> DSSDEASVSPIADNEREAVTLLLGYLEDKDQLDFYSGGPLKALTTLVYSDNLNLQRSAALAFAEITEKYVRQVSREVLEPILILLQSQDPQIQVAACAALGNLAVNNENKLLIVEMGGLEPLINQMMGDNVEVQCNAVGCITNLATRDDNKHKIATSGALIPLTKLAKSKHIRVQRNATGALLNMTHSEENRKELVNAGAVPVLVSLLSSTDPDVQYYCTTALSNIAVDEANRKKLAQTEPRLVSKLVSLMDSPSSRVKCQATLALRNLASDTSYQLEIVRAGGLPHLVKLIQSDSIPLVLASVACIRNISIHPLNEGLIVDAGFLKPLVRLLDYKDSEEIQCHAVSTLRNLAASSEKNRKEFFESGAVEKCKELALDSPVSVQSEISACFAILALADVSKLDLLEANILDALIPMTFSQNQEVSGNAAAALANLCSRVNNYTKIIEAWDRPNEGIRGFLIRFLKSDYATFEHIALWTILQLLESHNDKVEDLVKNDDDIINGVRK;> GGNSSTSALNSRRNSLDKSSNKQGMSGLPPIFGGESTSYHHDNKIQKYNQLGVEE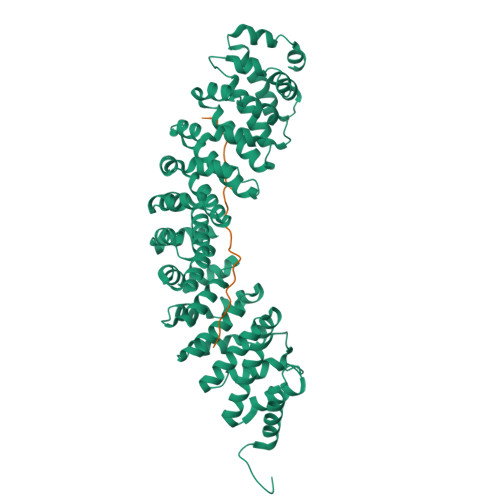DDDDENDRLLNQMGNSATKFKSSISPRSIDSISSSFIKSRIPIRQPYHYSQPTTAPFQAQAKFHKPANKLIDNG>[3x]MAHHHHHHSAALEVLFQGPGNNELSPVALRQMSCAAGTTQTACTDDNALAYYNTTKGGRFVLALLSDLQDLKW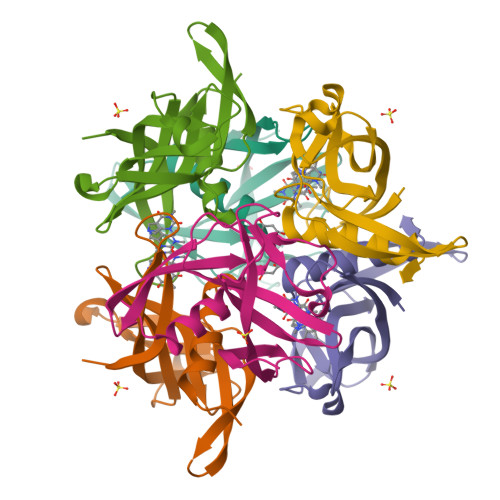ARFPKSDGTGTIYTELEPPCRFVTDTPKGPKVKYLYFIKGLNNLNRGMVLGSLAATVRLQ(2S,3aS,10Z,11aS,12aR)-2-({8-fluoro-7-methoxy-2-[4-(propan-2-yl)-1,3-thiazol-2-yl]quinolin-4-yl}oxy)-5-methyl-N-[(1-methylcyclopropyl)sulfonyl]-4,14-dioxo-1,2,3,3a,4,5,6,7,8,9,11a,12,13,14-tetradecahydro-12aH-cyclopropa[m]pyrrolo[1,2-c][1,3,6]triazacyclotetradecine-12a-carboxamide | C37 H45 F N6 O7 S2 | 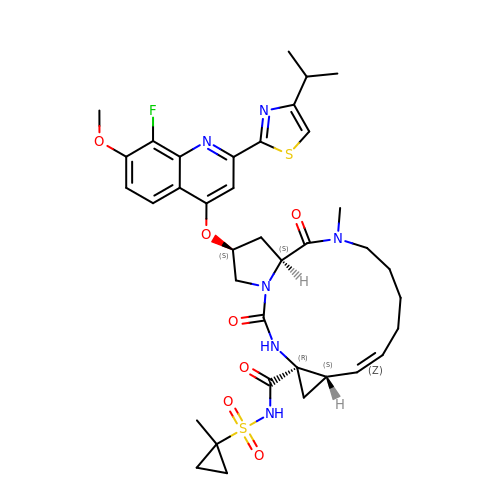WCUAGYIETHEUQO-MULYSJGUSA-N(1S)-1-(4-oxo-5-phenyl-3,4-dihydrothieno[2,3-d]pyrimidin-2-yl)ethyl [(2S)-3-oxo-3,4-dihydro-2H-1,4-benzothiazin-2-yl]acetate | C24 H19 N3 O4 S2 | 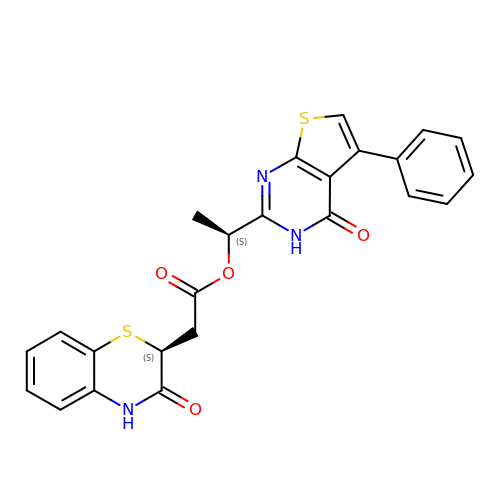KTBNGJHCLCHCKH-UGSOOPFHSA-N> MSLKLTPEAAGTFAIAPTPFHDDGKIDDVSIDRLTDFYAEVGCEGVTVLGILGEAPKLDAAEAEAVATRFIKRAKSMQVIVGVSAPGFAAMRRLARLSMDAGAAGVMIAPPPSLRTDEQITTYFRQATEAIGDDVPWVLQDYPLTLSVVMTPKVIRQIVMDSASCVMLKHEDWPGLEKITTLRGFQKDGSLRPLSILCGNGGLFLDFEMERGADGAMTGYCFPDMLVDVVKLSKAGQRDLAHNLFDAHLPLIRYEHQQGVGLSVRKYVLKKRGLLSSSAQRKP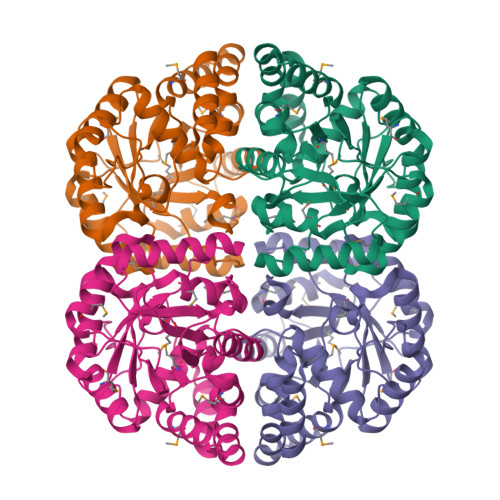GASLTDTAREEVDYLLSRLARVEGHHHHHH> MASLEDGTYRLRAVTTHNPDPGVGGEYATVEGARQPVKAEPSTPPFSEQQIWQVTRNSDGQYTIKYQGLNAPFEYGFSYDQLEPNAPVIAGDPKEYILQLVPSTADVYIIRAPIQRVGVDVEVGVQGNTLVYKFFPVDGSGGDRPAWRFT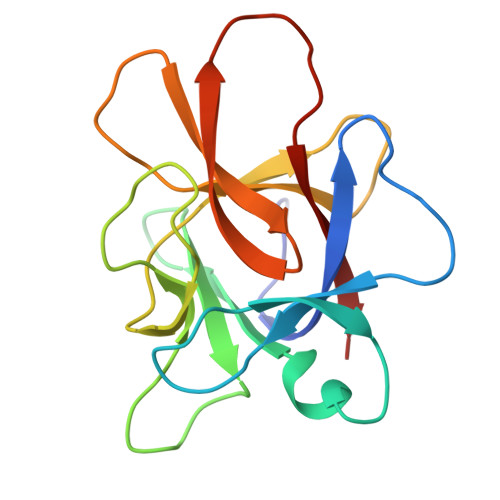RE>MAEKPKLHYFNARGRMESTRWLLAAAGVEFEEKFIKSAEDLDKLRNDGYLMFQQVPMVEIDGMKLVQTRAILNYAASKYNLYGKDIKERALIDMYIEGIADLGEMILLLPVCPPEEKDAKLALIKEKIKNRYFPAFEKVLKSHGQDYLVGNKLSRADIHLVELLYYVEELDSSLISSFPLLKALKT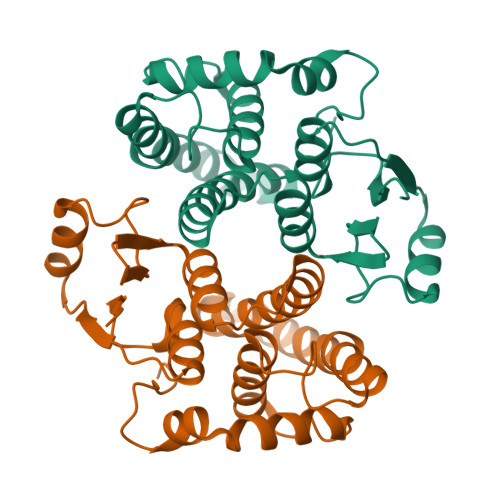RISNLPTVKKFLQPGSPRKPPMDEKSLEEARKIFRF[2x]>[2x]MKRVSRRAFLRRLGVGVAATAAFSPLAVAQARRYRWRIQTAWDAGTVGYSLFQKFTERVKELTDGQLEVQPFPAGAVVGTFDMFDAVKTGVLDGMNPFTLYWAGRMPVTAFLSSYALGLDRPDQWETWFYSLGGLDIAR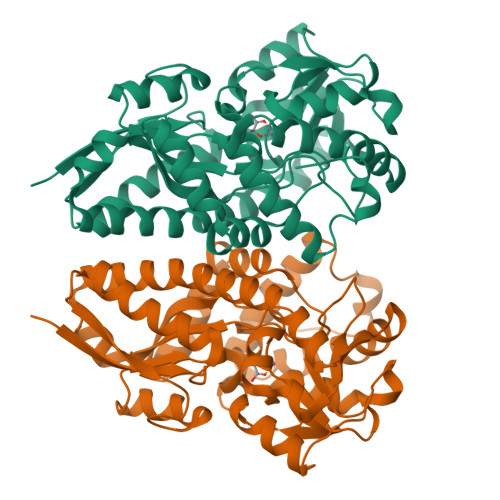RAFAEQGLFYVGPVQHDLNIIHSKKPIRRFEDFKGVKLRVPGGMIAEVFAAAGASTVLLPGGEVYPALERGVIDAADFVGPAVNYNLGFHQVAKYIIMGPPETPAIHQPVDLMDFTINLNRWRSLPKPLQERFIAAVHEYSWIHYAGIQKANLEAWPKYRQAGVEVIRLSNEDVRKFRRLAIPIWFKWAKMDKYSREAFASQLEYMKGIGYVTDEELKGLSL>[2x]GKEQPQVRGELEETQETQEDGNSTQRTTPVSVNYHFTRQCNYKCGFCFHTAKTSFVLPLEEAKRGLLLLKQAGLEKINFSGGEPFLQDRGEYLGKLVRFC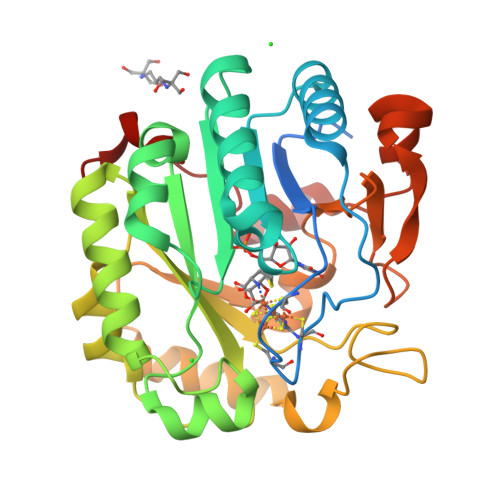KEELALPSVSIVSNGSLIRERWFKDYGEYLDILAISCDSFDEQVNALIGRGQGKKNHVENLQKLRRWCRDYKVAFKINSVINRFNVDEDMNEHIKALSPVRWKVFQCLLIEGENSGADALRAAERFLISNEEFETFLERHKEVSCLVPESNQKMKDSYLILDEYMRFLNCTGGRKDPSKSILDVGVEEAIKFSGFDEKMFLKRGGKYVWSKADLKLDW>[2x]ACDYTCGSNCYSSSDVSTAQAAGYKLHEDGETVGSNSYPHKYNNYEGFDFSVSSPYYE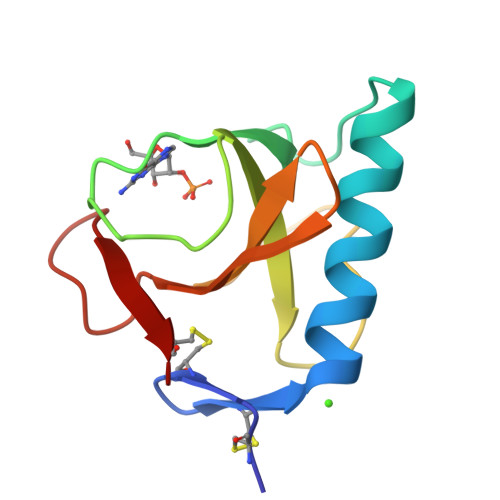YPILSSGDVYSGGSPGADRVVFNENNQLAGVITHTGASGNNFVECT>[2x]MKSVITTTISAADAAGRFPSSS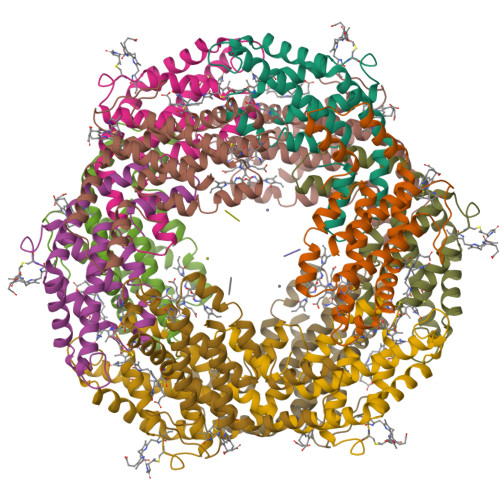DLESIQGNIQRAAARLEAAQKLSGNHEAVVKEAGDACFAKYSYLKNAGEAGDSPEKINKCYRDIDHYMRLINYSLVVGGTGPVDEWGIAGSREVYRALNLPGSAYIAAFTFTRDRLCVPRDMSSQAGVEFTSALDYVINSLC;>[2x]MLDAFSRVVVTSDAKAAYVGGSDLQSLKSFINDGNKRLDAVNYIVSNASCIVSDAVSGMICENPGLIAPGGNCYTNRRMAACLRDGEIILRYVSYALLAGDSSVLDDRCLNGLKETYIALGVPTASSSRAVSIMKATATAFITNTASGRKVEVAAGDCQALQAEAASYFDKVGSSID>MPGVRGQVDKQVSTAIENIENKLVASGPGVTRYLTLPQTGWTPEQIRTELDKLANMEHTRWEDGRVSGAVYHGGQDLLKLQTEAFGQFGVANPIHPDVFPGVRKMEAEVVAMVLALFNAPSDGAGVTTSGGTESILMACLAARQKAFTERGVKEPEIIIPDTAHAAFYKACNYFGMKLHRVPCPAPEYKVDIAAVRRLINPNTVLLVGSAPNFPHGIVDDIPALSRLATKYKIPLHVDCCLGSFVIAFLKKAGFPSPYEEEGGFDFRLPGVTSISVDTHKYGFAPKGNSVLLYRNKTYRSYQYFIYPDWSGGVYASPSVAGSRPGALIAGCWASLMSVGETGYINSCLEIIGAAKKFEASIKEHPVLSKNLGIVGKPMVSVVAFQSQNGAVDIYDVADGLSAKGWHLNALQSPPAIHVAFTIPTAAAVEKLTTDLVETVEKELEKAEERKRQGKSYVLKRGDTSALYGVAGSLPDKSIVSRLAEGFLDT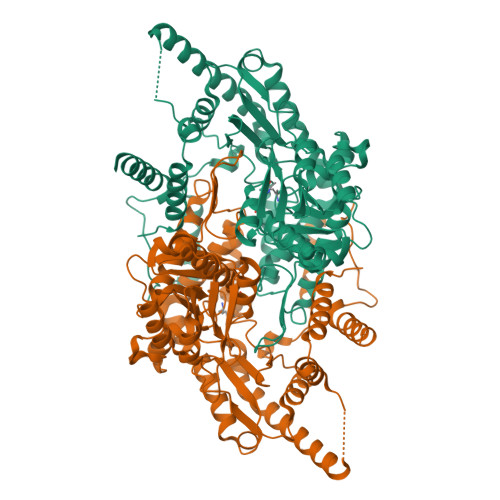LYKAGGGSHHHHHH[2x]>[6x]MAPTKRKGECPGAAPKKPKEPVQVPKLLIKGGVEVLEVKTGVDAITEVECFLNPEMGDPDENLRGFSLKLSAENDFSSDSPERKMLPCYSTARIPLPNLNEDLTCGNLLMWEAVTVQTEVIGITSMLNLHAGSQKVHEHGGGKPIQGSNFHFFAVGGEPLEMQGVLMNYRSKYPDGTITPKNPTAQSQVMNTDHKAYLDKNNAYPVECWVPDPSRNENARYFGTFTGGENVPPVLHVTNTATTVLLD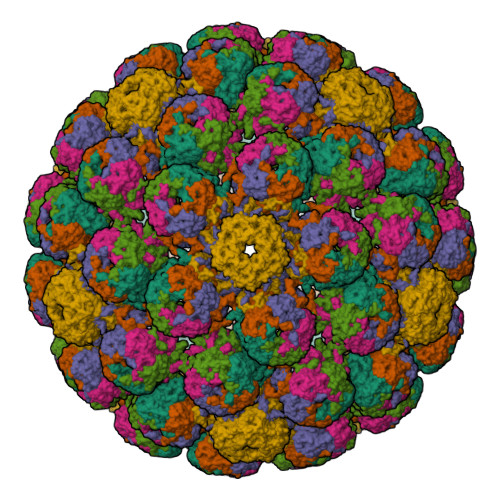EQGVGPLCKADSLYVSAADICGLFTNSSGTQQWRGLARYFKIRLRKRSVKNPYPISFLLSDLINRRTQRVDGQPMYGMESQVEEVRVFDGTERLPGDPDMIRYIDKQGQLQTKML4,4'-(1H-1,2,3-triazole-1,5-diyl)diphenol | C14 H11 N3 O2 | 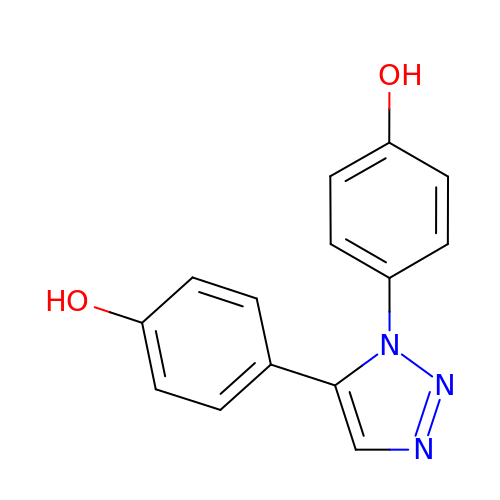VJAKQEJLSICLIC-UHFFFAOYSA-N> AYPNWDKLLKKYNQGQLSIEDLLKIHSSTNERVATLNDFYTYVFGNIKHVSSILDFGCGFNPLALYQWNENEKIIYHAYDIDRAEIAFLSSIIGKLKTTIKYRFLN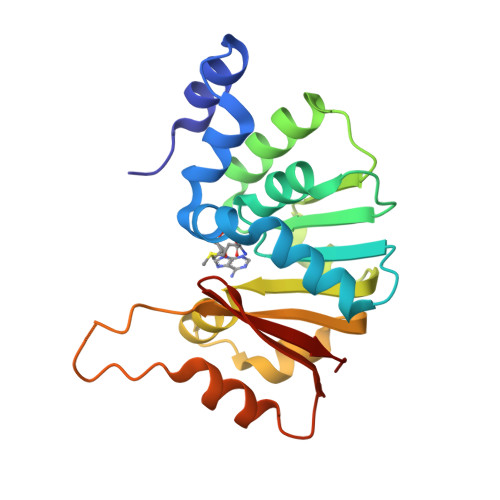KESDVYKGTYDVVFLLKMLPVLKQQDVNILDFLQLFHTQNFVISFPIKSLSGKEKGMEENYQLWFESFTKGWIKILDSKVIGNELVYITSGFQK> IETVPVKLKPGMDGPKVKQWPLTEEKIKALVEICTEMEKEGKISKIGPENPYNTPVFAIKKKDSTKWRKLVDFRELNKRTQDFWEVQLGIPHPAGIKKKKSVTVLDVGD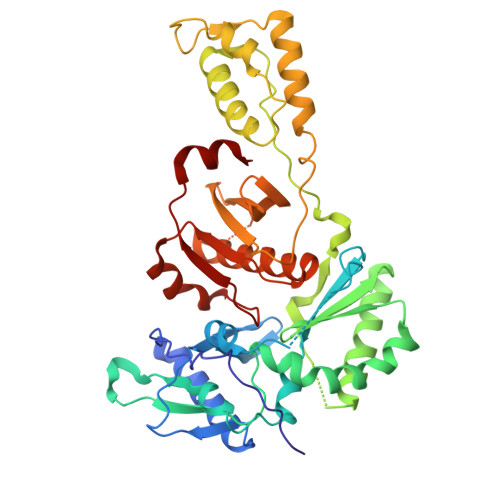AYFSVPLDEDFRKYTAFTIPSINNETPGIRYQYNVLPQGWKGSPAIFQSSMTKILEPFRKQNPDIVIYQYMDDLYVGSDLEIGQHRTKIEELRQHLLRWGLTTPDKKHQKEPPFLWMGYELHPDKWTVQPIVLPEKDSWTVNDIQKLVGKLNWASQIYPGIKVRQLCKLLRGTKALTEVIPLTEEAELELAENREILKEPVHGVYYDPSKDLIAEIQKQGQGQWTYQIYQEPFKNLKTGKYARMRGAHTNDVKQLTEAVQKITTESIVIWGKTPKFKLPIQKETWETWWTEYWQATWIPEWEFVNTPPLVKLWYQ> GCTGGATATATCCAGC

The rational design of small molecules that target specific DNA sequences is a promising strategy to modulate gene expression. This report focuses on a diamidinobenzimidazole compound, whose selective binding to the minor groove of AT DNA sequences holds broad significance in the molecular recognition of AT-rich human promoter sequences. The specialized method of X-ray crystallography was utilized to investigate how the sequence-dependent recognition properties in general, A-tract, and alternating AT sequences affect the binding of diamidinobenzimidazole in the DNA minor groove. A strong and direct hydrogen bond between the N-H of the benzimidazole and an H-bond acceptor atom in the minor groove is essential for DNA recognition in all sequences described. In addition, the diamidine compound specifically utilizes an interfacial water molecule for its DNA binding.

Our experiments to additionally investigate the minor groove of alternating AT DNA sequences using d(5′-GCTGGATATATCCAGC-3′)2 resulted in a structure with a narrow minor groove width similar to that of the dodecameric structure. In this report, we show the two native alternating AT DNAs,16-mer ATATAT and 12-mer ATAT, to have a narrow minor groove. Overall, the many reports regarding alternating AT sequences lead us to conclude that ATATAT DNA crystal structures can have both wide and narrow minor grooves depending on the experimental crystallization conditions and local packing interactions.> MNIVVCIKQVPDTTEVKLDPNTGTLIRDGVPSIINPDDKAGLEEAIKLKEEMGAHVTVITMGPPQADMALKEALAMGADRGILLTDRAFAGADTWATSSALAGALKNIDFDIIIAGRQAIDGDTAQVGPQIAEHLNLPSITYAEEIKTEGEYVLVKRQFEDCCHDLKVKM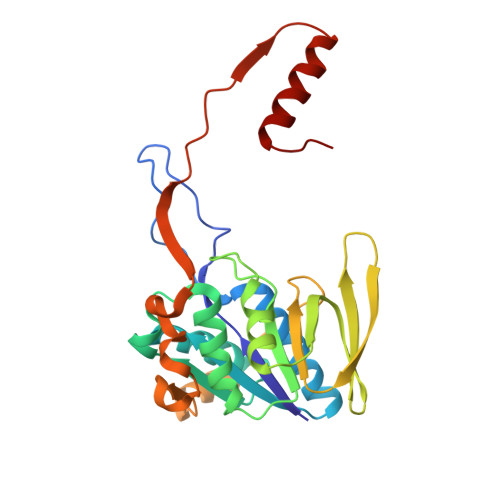PCLITTLKDMNTPRYMKVGRIYDAFENDVVETWTVKDIEVDPSNLGLKGSPTSVFKSFTKSVKPAGTIYNEDAKTSAGIIIDKLKEKYII> VLSSLRMAAILDDQTVCGRGERLALALAREQINGIIEVPAKARVEVDIFELQRDSQYETTDTMCQILPKGVVSVLGPSSSPASASTVSHICGEKEIPHIKVGPEETPRLQYLRFASVSLYPSNEDVSLAVSRILKSFNYPSASLICAKAECLLRLEELVRGFLISKETLSVRMLDDSRDPTPLLKEIRDDKVSTIIIDANASISHLVLRKASELGMTSAFYKYILTTMDFPILHLDGIVEDSSNILGFSMFNTSHPFYPEF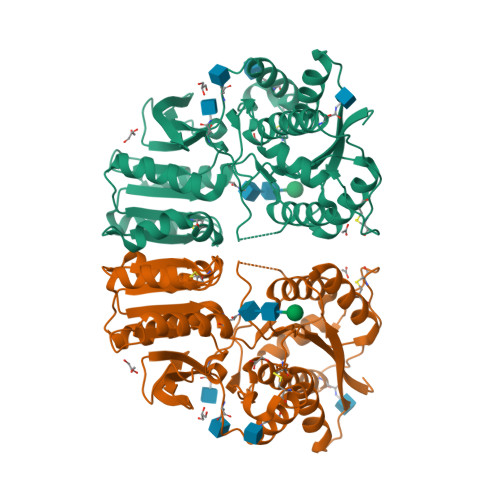VRSLNMSWRENCEASTYPGPALSAALMFDAVHVVVSAVRELNRSQEIGVKPLACTSANIWPHGTSLMNYLRMVEYDGLTGRVEFNSKGQRTNYTLRILEKSRQGHREIGVWYSNRTLAMNATTLDILELVPR> MKGKMAIVISTLNNPWFVVLAETAKQR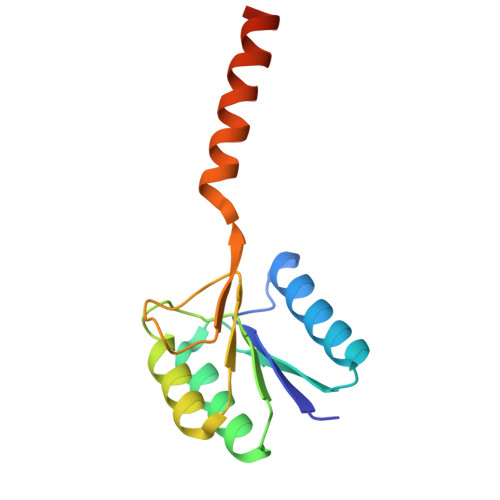AEQLGYEATIFDSQNDTAKESAHFDAIIAAGYDAIIFNPTDADGSIANVKRAKEAGIPVFCVDRGINARGLAVAQIYSDNYYGGVLMGEYFVKFLKEKKLEHHHHHH>[8x]GHMASRAEEGLNFPTYDGKDRVVSLSEKNFKQVLKKYDLLCLYYHEPVSSDKVTQKQFQLKEIVLELVAQVLEHKAIGFVMVDAKKEAKLAKKLGFDEEGSLYILKGDRTIEFDGEFAADVLVEFLLDLIEDPVEIISSKLEVQAFERIEDYIKLIGFFKSEDSEYYKAFEEAAEHFQPYIKFFATFDKGVAKKLSLKMNEVDFYEPFMDEPIAIPNKPYTEEELV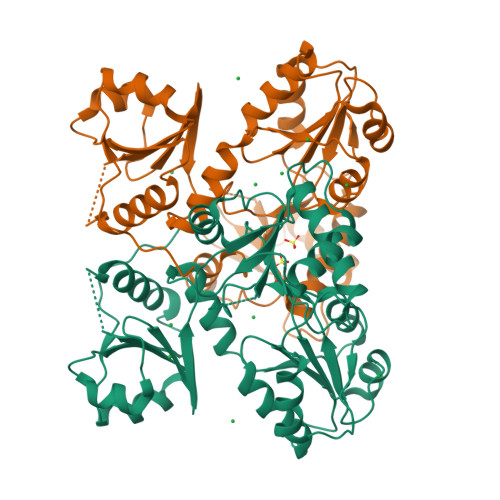EFVKEHQRPTLRRLRPEEMFETWEDDLNGIHIVAFAEKSDPDGYEFLEILKQVARDNTDNPDLSILWIDPDDFPLLVAYWEKTFKIDLFRPQIGVVNVTDADSVWMEIPDDDDLPTAEELEDWIEDVLSGKINTEDDDEDDDDDDNSDEEDNDDSDDDDDE> MVPISPIETVPVKLKPGMDGPKVKQWPLTEEKIKALVEICTEMEKEGKISKIGPENPYNTPVFAIKKKDSTKWRKLVDFRELNKRTQDFWEVQLGIPHPAGLKQKKSVTVLDVGDAYFSVPLDKDFRKYTAFTIPSINNETPGIRYQYNVLPMGWKGSPAIFQSSMTKILEPFRKQNPDIVIYQYMDDLYVGSDL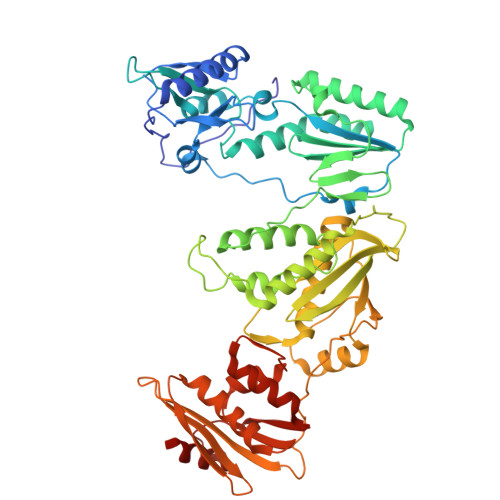EIGQHRTKIEELRQHLLRWGFTTPDKKHQKEPPFLWMGYELHPDKWTVQPIVLPEKDSWTVNDIQKLVGKLNWASQIYAGIKVRQLSKLLRGTKALTEVVPLTEEAELELAENREILKEPVHGVYYDPSKDLIAEIQKQGQGQWTYQIYQEPFKNLKTGKYARMKGAHTNDVKQLTEAVQKIATESIVIWGKTPKFKLPIQKETWEAWWTEYWQATWIPEWEFVNTPPLVKLWYQLEKEPIIGAETFYVDGAANRETKLGKAGYVTDRGRQKVVPLTDTTNQKTELQAIHLALQDSGLEVNIVTDSQYALGIIQAQPDKSESELVSQIIEQLIKKEKVYLAWVPAHKGIGGNEQVDKLVSAG> SDAHDEETFEEFTARYEKEFDEAYDLFEVQ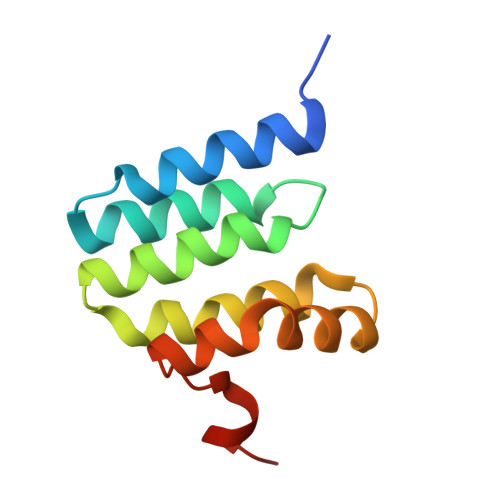RVLNNCFSYDLVPAPAVIEKALRAARRVNDLPTAIRVFEALKYKVENEDQYKAYLDELKDVRQELGVPLKEELFPSSS>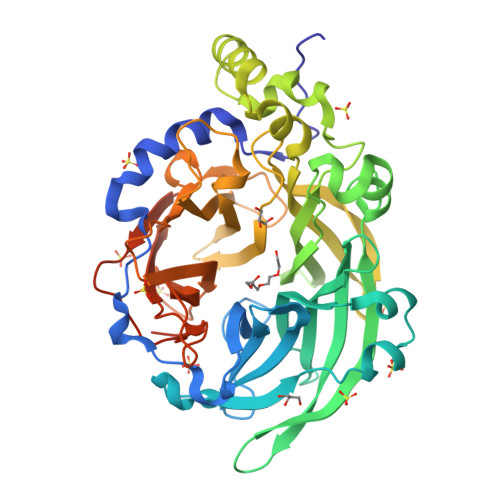[2x]KETNQKPYKETYGISHITRHDMLQIPEQQKNEKYQVPEFDSSTIKNISSAKGLDVWDSWPLQNADGTVANYHGYHIVFALAGDPKNADDTSIYMFYQKVGETSIDSWKNAGRVFKDSDKFDANDSILKDQTQEWAGSATFTSDGKIRLFYTDFSGKHYGKQTLTTAQVNVSASDSSLNINGVEDYKSIFDGDGKTYQNVQQFIDEGNYSSGDNHTLRDPHYVEDKGHKYLVFEANTGTEDGYQGEESLFNKAYYGKSTSFFRQESQKLLQSDKKRTAELANGALGMIELNDDYTLKKVMKPLIASNTVTDEIERANVFKMNGKWYLFTDSRGSKMTIDGITSNDIYMLGYVSNSLTGPYKPLNKTGLVLKMDLDPNDVTFTYSHFAVPQAKGNNVVITSYMTNRGFYADKQSTFAPSFLLNIKGKKTSVVKDSILEQGQLTVNKTDPNSSSVDKLAAALEHHHHHH> MPSALAIFTCRPNSHPFQERHVYLDEPIKIGRSVARCRPAQNNATFDCKVLSRNHALVWFDHKTGKFYLQDTKSSNGTFINSQRLS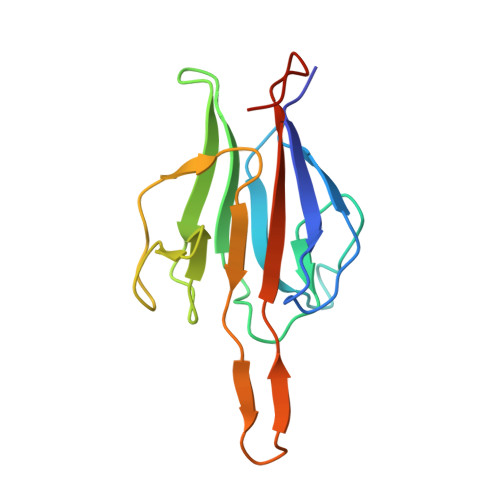RGSEESPPCEILSGDIIQFGVDVTENTRKVTHGCIVSTIKLFLPDGMEARLRSD> MKVEEILEKALELVIPDEEEVRKGREAEEELRRRLDELGVEYVFVGSYARNTWLKGSLEIDVFLLFPEEFSKEELRERGLEIGKAVLDSYEIRYAEHPYVHGVVKGVEVDVVPCYKLKEPKNIKSAVDRTPFHHKWLEGRIKGKENEVRLLKGFLKANGIYGAEYKVRGFSGYLCELLIVFYGSFLETVKNARRWTRRTVIDVAKGEVRKGEEFFVVDPVDEKRNVAANLSLDNLARFVHLCREFMEAPSLGFFKPKHPLEIEPERLRKIVEERGTAVFAVKFRKPDIVDDNLYPQLERASRKIFEFLERENFMPLRSAFKASEEFCYLLFECQIKEISRVFRRMGPQFEDERNVKKFLSRNRAFRPFIENGRWWAFEMRKFTTPEEGVRSYASTHWHTLGKNVGESIREYFEIISGEKLFKEPVTAELCEMMGVKDCCCM;> MKVEEILEKALELVIPDEEEVRKGREAEEELRRRLDELGVEYVFVGSYARNTWLKGSLEIDVFLLFPEEFSKEELRERGLEIGKAVLDSYEIRYAEHPYVHGVVKGVEVDVVPCYKLKEPKNIKSAVDRTPFHHKWLEGRIKGKENEVRLLKGFLKANGIYGAEYKVRGFSGYLCELLIVFYGSFLETVKNARRWTRRTVIDVAKGEVRKGEEFFVVDPVDEKRNVAANLSLDNLARFVHLCREFMEAPSLGFFKPKHPLEIEPERLRKIVEERGTAVFAVKFRKPDIVDDNLYPQLERASRKIFEFLERENFMPLRSAFKASEEFCYLLFECQIKEISRVFRR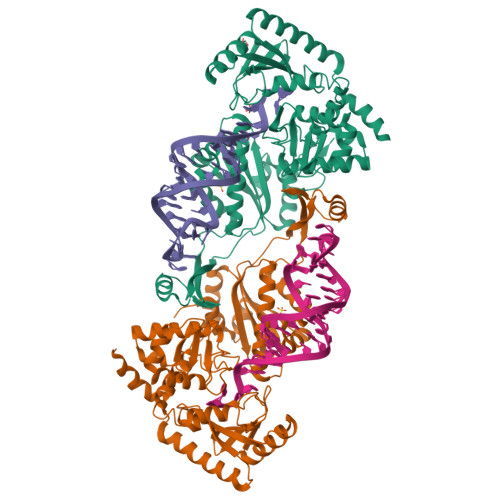MGPQFEDERNVKKFLSRNRAFRPFIENGRWWAFEMRKFTTPEEGVRSYASTHWHTLGKNVGESIREYFEIISGEKLFKEPVTAELCEMMGVKD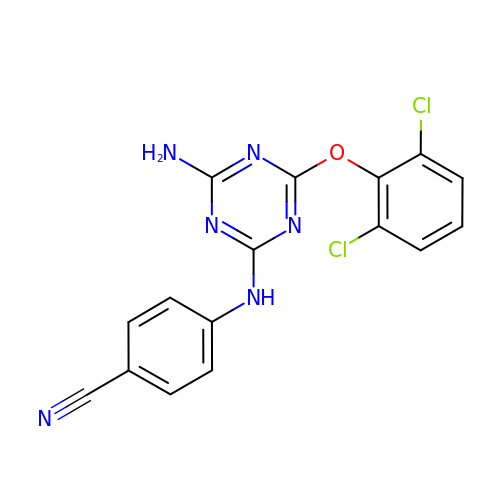4-[4-AMINO-6-(2,6-DICHLORO-PHENOXY)-[1,3,5]TRIAZIN-2-YLAMINO]-BENZONITRILE | C16 H10 Cl2 N6 O | NFNNMVVXXITVGD-UHFFFAOYSA-N> GSLVLYGAPYERAVEVLEETLRETGARYALLIDRKGFVLAHKEALWAPKPPPLDTLATLVASNAAATQALAKLLGEARFQEEVHQGERM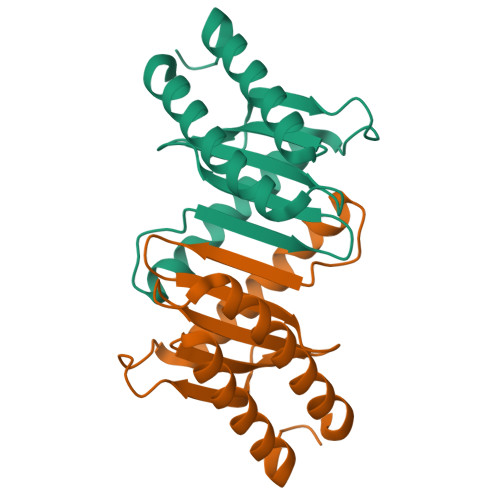GLYVDEAGEHALLVLVFDETAPLGKVKLHGKRAAEALARIAEEALAN> MDAVAVYHGKISRETGEKLLLATGLDGSYLLRDSESVPGVYC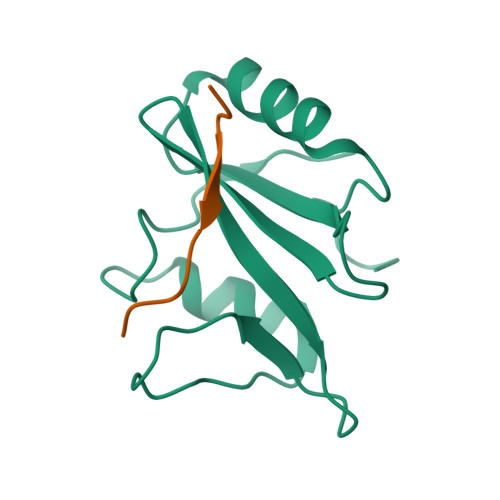LCVLYHGYIYTYRVSQTETGSWSAETAPGVHKRYFRKIKNLISAFQKPDQGIVIPLQYPVEK;> KSLTIYAQVQK>[3x]GAMDHVEFMSASKEIKSFLWTQSLRRELSGYCSNIKLQVVKDAQALLHGLDFSEVSNVQRLMRKERRDDNDLKRLRDLNQAVNNLVELKSTQQKSILRVGTLTSDDLLILAADLEKLKSKVIRTERPLSAGVYMGNLSSQQLDQRRALLNMIGMSGGNQGAR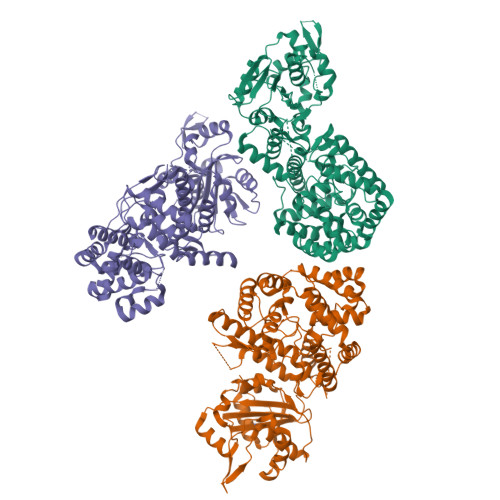AGRDGVVRVWDVKNAELLNNQFGTMPSLTLACLTKQGQVDLNDAVQALTDLGLIYTAKYPNTSDLDRLTQSHPILNMIDTKKSSLNISGYNFSLGAAVKAGACMLDGGNMLETIKVSPQTMDGILKSILKVKKALGMFISDTPGERNPYENILYKICLSGDGWPYIASRTSITGRAWENTVVDLESDGKPQKADSNNSSKSLQSAGFTAGLTYSQLMTLKDAMLQLDPNAKTWMDIEGRPEDPVEIALYQPSSGCYIHFFREPTDLKQFKQDAKYSHGIDVTDLFATQPGLTSAVIDALPRNMVITCQGSDDIRKLLESQGRKDIKLIDIALSKTDSRKYENAVWDQYKDLCHMHTGVVVEKKKRGGKEEITPHCALMDCIMFDAAVSGGLNTSVLRAVLPRDMVFRTSTPRVVL> MSSFIQYEFLKIYQGNQKIKNYYKRKRLIFQQKKVLKKKQKEIQMSTNNLRLKPWFHWTDEERSHAIFSAYEKRILKSEDLPSFLRANRINNVSTWVFPLIAL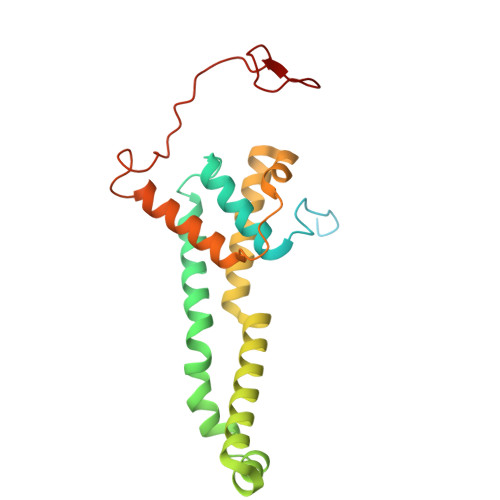PLFNQSIFKLGFAQRILLTRPAIEWHCFKIATVAASWLAWLNFSPFYRKLENEKEYLLDTLESRIGINVLDLNDALPRWTTSQEYNRRTQQLYNQRNGFFAGLLYPQEESSRPLVDIASFPKNLHKEKLTK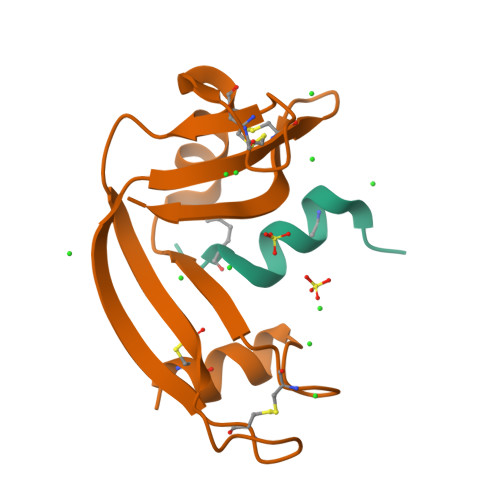> KETAASKFERQHLDS;> SSSNYCNQMMKSRNLTKDRCKPVNTFVHESLADVQAVCSQKNVACKNGQTNCYQSYSTMSITDCRETGSSKYPNCAYKTTQANKHIIVACEGNPYVPVHFDASV>[3x]GPGSMQWAVGR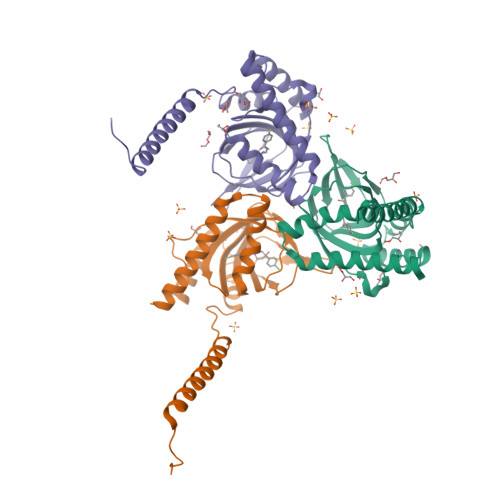RWAWAALLLAVAAVLTQVVWLWLGTQSFVFQREEIAQLARQYAGLDHELAFSRLIVELRRLHPGHVLPDEELQWVFVNAGGWMGAMCLLHASLSEYVLLFGTALGSRGHSGRYWAEISDTIISGTFHQWREGTTKSEVFYPGETVVHGPGEATAVEWGPNTWMVEYGRGVIPSTLAFALADTVFSTQDFLTLFYTLRSYARGLRLELTTYLFGQDP>MMSDQENENEHAKAFLGLAKCEEEVDAIEREVELYRLNKMKPVYEKRDAYI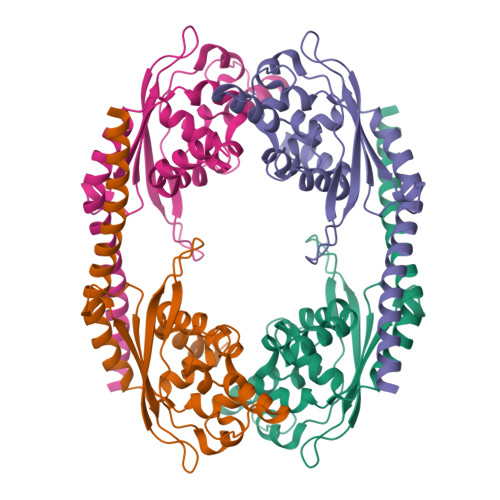DEIAEFWKIVLSQHVSFANYIRASDFKYIDTIDKIKVEWLALESEMYDTRDFSITFHFHGIEGDFKEQQVTKVFQIKKGKDDQEDGILTSEPVPIEWPQSYDSINPDLIKDKRSPEGKKKYRQGMKTIFGWFRWTGLKPGKEFPHGDSLASLFSEEIYPFCVKYYAEAQRDLEDEEGESGLSADGDSEDDDGSLGEVDLPLSDEEPSSKKRKV[4x]Serine O-acetyltransferase (CysE) is an enzyme in many bacteria that catalyzes the first step in l-cysteine biosynthesis by transferring an acetyl group from acetyl coenzyme A (acetyl-CoA) to l-serine to form O-acetylserine. Lack of the CysE/CysK-dependent l-cysteine biosynthesis pathway in mammals suggests that those bacterial enzymes may become targets for antimicrobial agents. In this study, we used recombinant CysE cloned from Salmonella Typhimurium (StCysE). Here, we demonstrated that alkyl gallates such as octyl gallate (OGA) could act as potent CysE inhibitors in vitro and in bacteria.

Because of the poor water solubility of OGA, we could not crystalize StCysE in a complex with OGA. We did, however, successfully obtain a co-crystal of StCysE complexed with BGA and hence could determine its crystal structure. BGA binds to the hydrophobic pocket of StCysE where it is very close to the binding site of CoA. The hydroxyl group of BGA interacts with the main chain O atom of Gly-184 and the main chain O atom of Ile-220. The ketone group of BGA interacts with the side chain of Lys-219. The ester O atom of BGA interacts with the main chain N atom of Ala-222. The hydrophobic alkyl chain of BGA is surrounded by hydrophobic residues of the enzyme: Leu-209, Ala-222, Leu-227, and Ala-237. The binding site of acetyl-CoA overlaps with the BGA-binding site. Thus, binding of BGA to the enzyme may compete with binding of acetyl-CoA, which would result in inhibition of StCysE activity. It should be note that all these amino acids that make up the binding site of butyl gallate are conserved between StCysE and EcCysE.

>[12x]MHHHHHHDPPCEELEIVWKNIKAEARALADCEPMLASFYHATLLKHENLGSALSYMLANKLASPIMPAIAIREVVEEAYAADPEMIASAACDIQAVRTRDPAVDKYSTPLLYLKGFHALQAYRIGHWLWNKGRRALAIFLQNQVSVSFQVDIHPAAKIGRGIMLDHATGIVVGETAVIEDDVSILQSVTLGGTGKTSGDRHPKIREGVMIGAGAKILGNIEVGRGAKIGAGSVVLQPVPPHTTAAGVPARIVGKPGSDKPSMDMDQHFNGIHHTFEYGDG>MSEDNFDDEFDGSLPSGPRHPMARRFRGYLPVVVDVETGGFNSATDALLEIAATTVGMDEKGFLFPEHTYFFRIEPFEGANIEPAALEFTGIKLDHPLRMAVQEEAALTEIFRGIRKALKANGCKRAILVGHNSSFDLGFLNAAVARTGIKRNPFHPFSSFDTATLAGLAYGQTVLAKACQAAGMEFD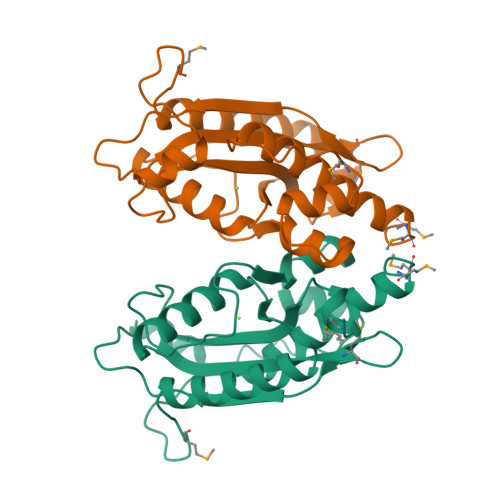NREAHSARYDTEKTAELFCGIVNRWKEMGGWMDDDD[2x]>RKPIIAGNWKMNGTLAEAVQFVEDVKGHVPPADEVISVVCAPFLFLDRLVQAADGTDLKIGAQTMHFADQGAYTGEVSPVMLKDLGVTYVILGHSERRQMFAETDETVNKKVLAAFTRGLIPIICCGESLEEREAG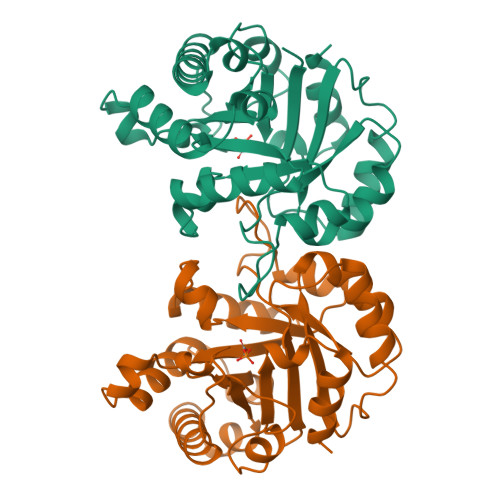QTNAVVASQVEKALAGLTPEQVKQAVIAYEPIWAIGTGKSSTPEDANSVCGHIRSVVSRLFGPEAAEAIRIQYGGSVKPDNIRDFLAQQQIDGALVGGASLEPASFLQLVEAGRHE[2x]> MRDLVRSGKVFLYGEFIGLLREDHRGFHFSYNPDY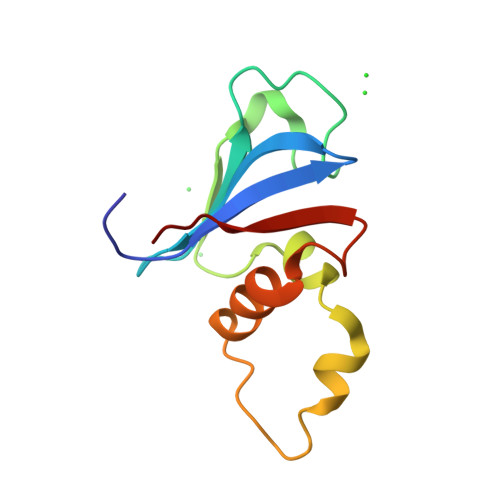QGIPLSLSFPIEQSPFHSDTLFPYFASLVPEGWLKHKYALHQRIDESDMFRFLLNNGENMLGAVQIQEEKQ> MSKAELAAMSEAEFRALLQGKKETLKNIIKELDEKIKELLEEHPDLSLEEKLAELLRFFVEVFSKNFSPEAAVTFYQNFYELLRTYAAVLHGEEAVPPPLVMTPELAAEIIALFQAATESEEGLEAFIAFVLGDPALQKLIDMLGKDKVVILSLFAIAFIKTAVDSALEEADKLGAAA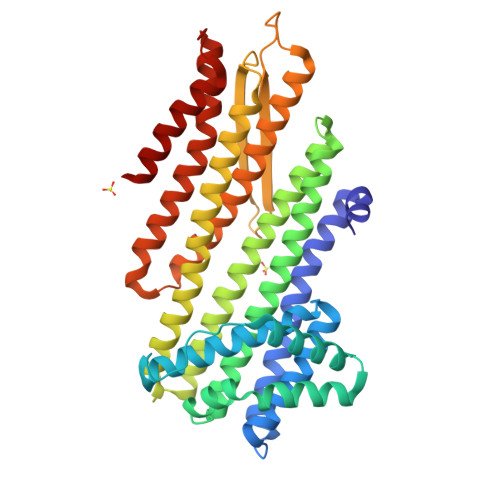LELAEENRGTAEGERHLQFYAATQGLKAWLKELEITETTKIFDDLIEERPELAAELEAVRDRVMGALLDEVLAEVDATVAAVLARLRALAEALDPKVRLTSVAVEVAWTEDGLLTVTVDVRTESGPLGATPEEIAEAQWAISRLLATAAAELSALERVLETLLKHVAEADKARVEAALARVETTRAGLIDIFREAAAAQAAGSPRTLAEIAAARLAALLAALAG> MASHKLLVTPPKALLKPLSIPNQLLLGPGPSNLPPRIMAAGGLQMIGSMSKDMYQIMDEIKEGIQYVFQTRNPLTL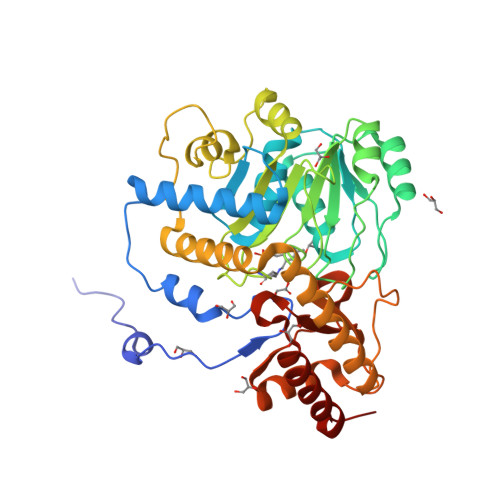VISGSGHCALEAALVNVLEPGDSFLVGANGIWGQRAVDIGERIGARVHPMTKDPGGHYTLQEVEEGLAQHKPVLLFLTHGESSTGVLQPLDGFRELCHRYKCLLLVDSVASLGGTPLYMDRQGIDILYSGSQKALNAPPGTSLISFSDKAKKKMYSRKTKPFSFYLDIKWLANFWGCDDQPRMYHHTIPVISLYSLRESLALIAEQGLENSWRQHREAAAYLHGRLQALGLQLFVKDPALRLPTVTTVAVPAGYDWRDIVSYVIDHFDIEIMGGLGPSTGKVLRIGLLGCNATRENVDRVTEALRAALQHCPKKKL>STPSIVIASAARTAVGSFNGAFANT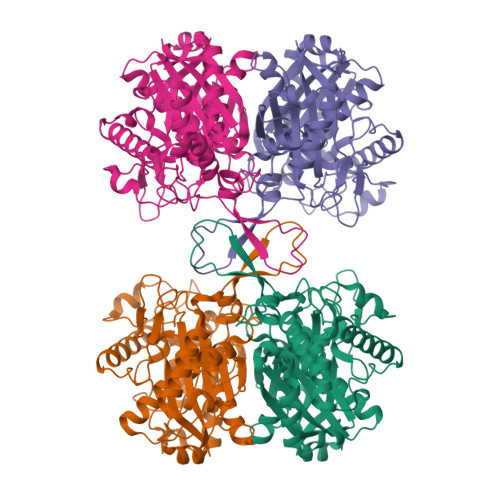PAHELGATVISAVLERAGVAAGEVNEVILGQVLPAGEGQNPARQAAMKAGVPQEATAWGMNQLCGSGLRAVALGMQQIATGDASIIVAGGMESMSMAPHCAHLRGGVKMGDFKMIDTMIKDGLTDAFYGYHMGTTAENVAKQWQLSRDEQDAFAVASQNKAEAAQKDGRFKDEIVPFIVKGRKGDITVDADEYIRHGATLDSMAKLRPAFDKEGTVTAGNASGLNDGAAAALLMSEAEASRRGIQPLGRIVSWATVGVDPKVMGTGPIPASRKALERAGWKIGDLDLVEAHEAFAAQACAVNKDLGWDPSIVNVNGGAIAIGNPIGASGARILNTLLFEMKRRGARKGLATLCIGGGMGVAMCIESL[4x]3-HYDROXYPENTANEDIOIC ACID | 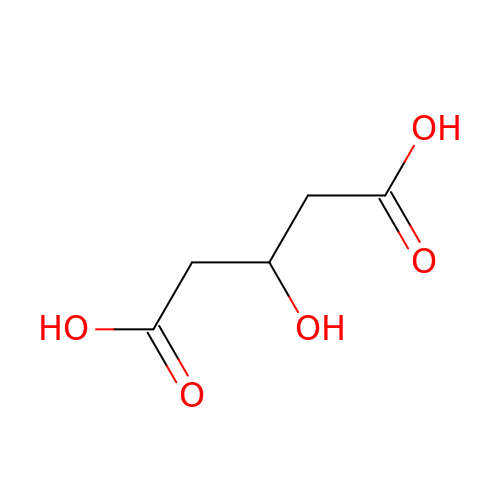C5 H8 O5 | ZQHYXNSQOIDNTL-UHFFFAOYSA-N>MNPAAEAEFNILLATDSYKVTHYKQYPPNTSKVYSYFECREKKTENSKLRKVKYEETVFYGLQYILNKYLKGKVVTKEKIQEAKDVYKEHFQDDVFNEKGWNYILEKYDGHLPIEIKAVPEGFVIPRGNVLFTVENTDPECYWLTNWIETILVQSWYPITVATNSREQKKILAKYLLETSGNLDGLEYKLHDFGYRGVSSQETAGIGASAHLVNFKRTDTVAGLALIKKYYGTKDPVPGYSVPAAEHSTITAWGKDHEKDAFEHIVTQFSSVPVSVVSDSYDIYNACEKIWGEDLRHLIVSRSTQAPLIIRPDSGNPLDTVLKVLEILGKKFPVTENSKGYKLLP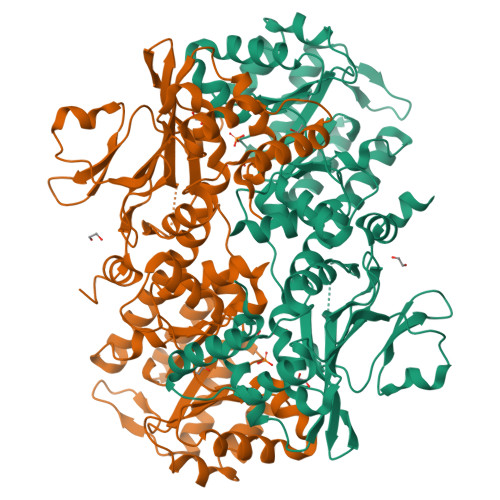PYLRVIQGDGVDINTLQEIVEGMKQKMWSIENIAFGSGGGLLQKLTRDLLNCSFKCSYVVTNGLGINVFKDPVADPNKRSKKGRLSLHRTPAGNFVTLEEGKGDLEEYGQDLLHTVFKNGKVTKSYSFDEIRKNAQLNIELEAAHHLEHHHHHHHH[2x]> SNEKIRSQSVLNTLETFFIKENHYDMQREESSIVNACLRYLGYSKSMCHEKMPIFMDIAFIEYCFNLSLDPSSFQNLPITQTQPDSQQILWEYSLISNALERLENIELERQNCMREDGLSKYTNSLLLNKETLNNEALKLYSCAKAGICRWMAFHFLEQEPIDHINFTKFLQDWGSHNEKEMEALQR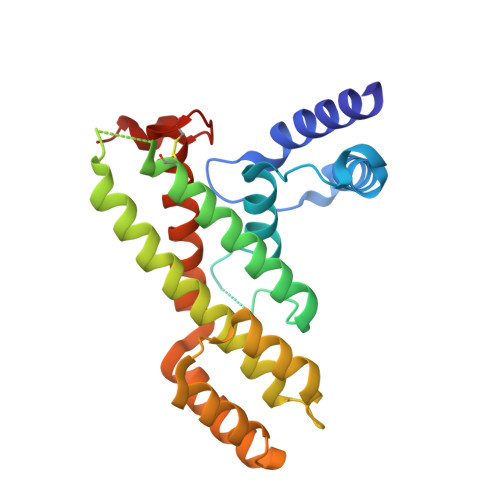LSKHKIRKRLIYVSQHKKKMPWSKFNSVLSRYIQCTKLQLEVFCDYDFKQREIVKMLTSNIN>[2x]SNAMLLYTKKDDIYSDIVRMILLIKGANAKIVDVSKEENSKHLEELNIITPNGNIPTLSTDDFAVYRLSVIIEAIEDLYPFPPMFPVFPKQRANARILLEYVNKTFLQNIIKLQSPDLDEKQANEIKMLMQRDIISTYKKIVSEREVNAESNPDAQNINVLTLIITFVFYYFIKLKISIPTKDKNIIKEIKELLSEPNFIKTIK;>SNAMVTLYTTKYCPYSLRARIALAEKKMSTDIVEAGDLEPAMIKKITPNGVFPVLMEKDYSINNRKALLIYIDERFPAPSLLPNVVNERIKIRLSLDKIDNEWYPVLDQIRKHRSDQKMLESMFKDLKESLLAMEKAFTGSEFFISSGFTLADCYIAALIICLEAEGFIIDDEYGAIYEYKKRLFARDSVKKANIKGGAGESLLKTLRTHR[2x]

An unusual set of Francisella regulators—the heteromeric macrophage growth locus protein A (MglA)–stringent starvation protein A (SspA) complex and the DNA-binding protein pathogenicity island gene regulator (PigR)—activates FPI transcription and thus is essential for virulence. The F. tularensis SspA protein, which shares ∼30% sequence identify with other bacterial SspAs, is not homodimeric and instead forms a complex with MglA. Multiple studies have shown that SspA proteins impart their function through interaction with RNA polymerase (RNAP), and, in Francisella, both MglA and SspA are required for RNAP interaction. Here we identify MglA–SspA as a novel ppGpp-binding complex and describe structures of apo- and ppGpp-bound MglA–SspA.

A previous study suggested that another small molecule involved in signaling, the inorganic polyphosphate hexametaphosphate (hexaMP), binds the MglA–SspA complex. However, we found that hexaMP did not compete with ppGpp binding to MglA–SspA. Moreover, cocrystallization of MglA–SspA with hexaMP revealed no electron density for this small molecule anywhere in the structure.> GSNKRLTEDERIEKELNTERQIFLEACIVRIMKAKRNLPHTTLVNECIAQSHQR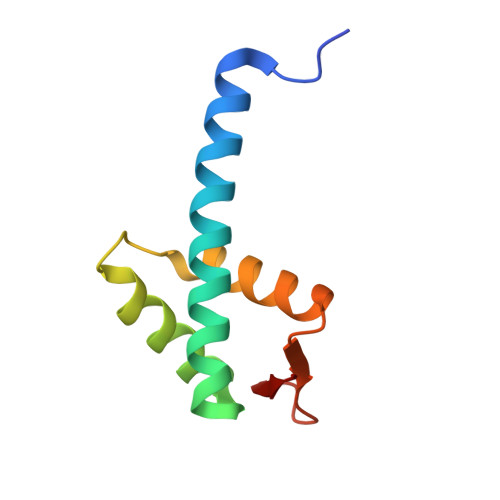FNAKVSMVKRAIDSLIQKGYLQRGDDGESYAYLA> SSGLNDIFEAQKIEWHEGSAGGSGGSGRSSLDNIEMAYARQIYIYNEKIVNGHLQPNLVDLCASVAELDDKSISDMWTMVKQMTDVLLTPATDALKNRSSVEVRMEFVRQALAYLEQSYKNYTLVTVFGNLHQAQLGGVPGTYQLVRSFLNIKLPAPLPGLQDGEVEGHPVWALIYYCMRCGDLLAASQVVNRAQHQLGEFKTWFQEYMNSKDRRLSPATENKLRLHYRRALRNNTDPYKRAVYCIIGRCDVTDNQSEVADKTEDYLWLKLNQVCFDDDGTSSPQDRLTLSQFQKQLLEDYGESHFTVNQQPFLYFQVLFLTAQFEAAVAFLFRMERLRCHAVHVALVLFELKLLLKSSGQSAQLLSHEPGDPPCLRRLNFVRLLMLYTRKFESTDPREALQYFYFLRDEKDSQGENMFLRCVSELVIESREFDMILGKLENDGSRKPGVIDKFTSDTKPIINKVASVAENKGLFEEAAKLYDLAKNADKVLELMNKLLSPVVPQISAPQSNKERLKNMALSIAERYRAQGISANKFVDSTFYLLLDLITFFDEYHSGHIDRAFDIIERLKLVPLNQESVEERVAAFRNF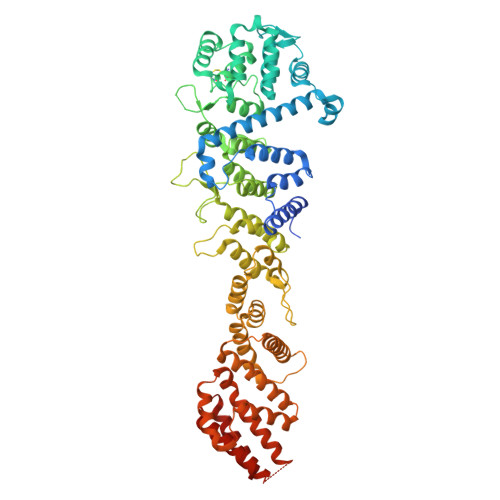SDEIRHNLSEVLLATMNILFTQFKRLKGTSPSSSSRPQRVIEDRDSQLRSQARTLITFAGMIPYRTSGDTNARLVQMEVLMN>MADPWQECMDYAVTLARQAGEVVCEAIKNEMNVMLKSSPVDLVTATDQKVEKMLISSIKEKYPSHSFIGEESVAAGEKSILTDNPTWIIDPIDGTTNFVHRFPFVAVSIGFAVNKKIEFGVVYSCVEGKMYTARKGKGAFCNGQKLQVSQQEDITKS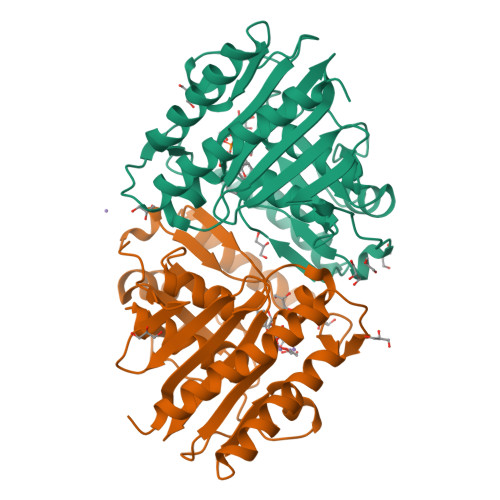LLVTELGSSRTPETVRMVLSNMEKLFCIPVHGIRSVGTAAVNMCLVATGGADAYYEMGIHCWDVAGAGIIVTEAGGVLMDVTGGPFDLMSRRVIAANNRILAERIAKEIQVIPLQRDDED[2x]>[4x]GMTESDRDYIQSIERGFAVLLAFDAQRPNPTLAELATEAGLSRPAVRRILLTLQKLGYVAGSGGRWSLTPRVLSIGQHYSESHALIEAAMPRLLEVAEKTQESASLGVLDGADVVYAARVPVRRIMSI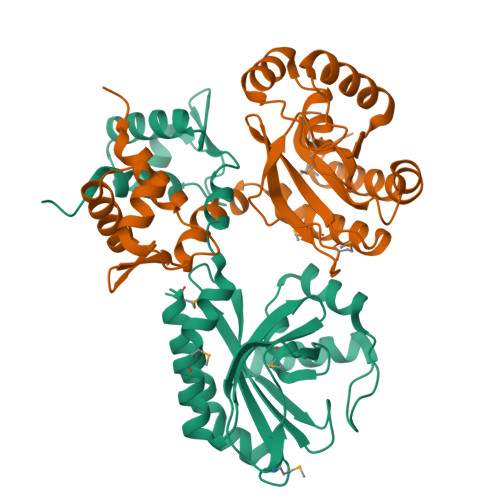NVSVGTRVPAYATSMGRALLAWAPADVVERVVAESTFQKLGPETIGTAAELERELAKVREQGFALTSEELEKGLISLAAPVHDAGGTVVGVVACSTSSARNTPAQFREQAVPCVLAAAAALSADMGFAG>[4x]MVISRAEIYWADLGPPSGSQPAKRRPVLVIQSDPYNASR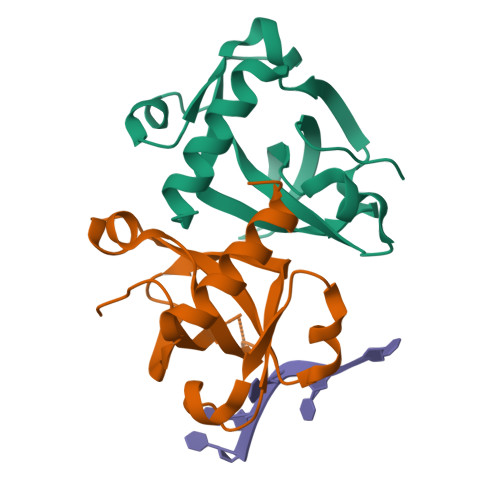LATVIAAVITSNTALAAMPGNVFLPATTTRLPRDSVVNVTAIVTLNKTDLTDRVGEVPASLMHEVDRGLRRVLDL L-HOMOARGININE | C7 H16 N4 O2 | 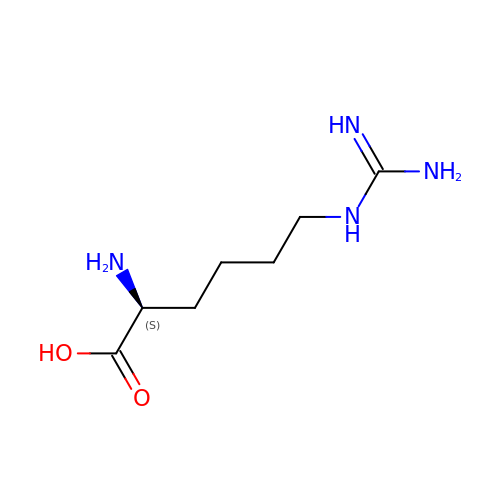QUOGESRFPZDMMT-YFKPBYRVSA-N(6R)-6-phenyl-1,3-thiazinane-2,4-dione 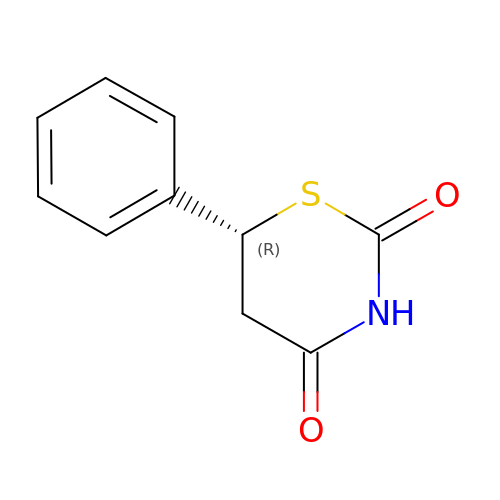| C10 H9 N O2 S | RYUNWBGPJCWGPJ-MRVPVSSYSA-N> MQIPASEQETLVRPKPLLLKLLKSVGAQKDTYTMKEVLFYLGQYIMTKRLYDEKQQHIVYCSNDLLGDLFGVPSFSVKEHR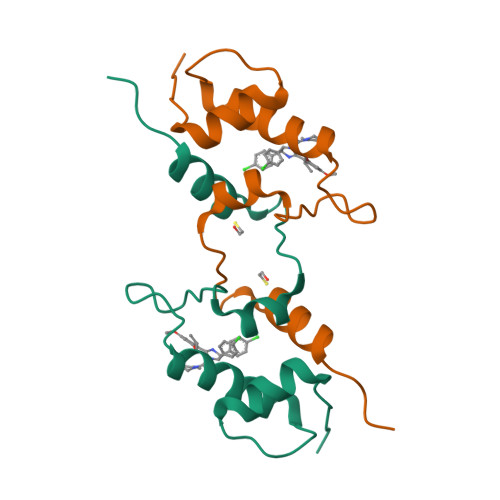KIYTMIYRNLVVVNQQ>[2x]RPMDNEAVQFGMSMGIGWNLGNQMDAHYDGCSYETGWGNKAATQQTFNG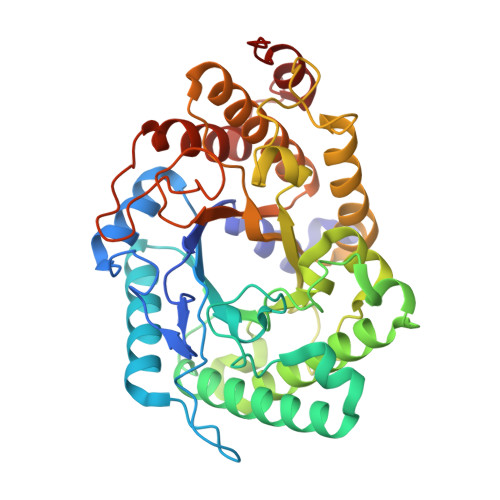LAKAGFRSVRIPVTWMGHIGNAPTYAIERGWLDRVDELVHMAHKAGLIVIINIHHDGFGAADTPSKGSHWLDLPAAVASEERNQLIKQELTMIWLQIGKRFANDGEWLVFETLNEIQDGDWGNGNNRRDGGAQYRVLNEWNQVCVDAIRAAGGKNETRYIGVPGYVCNPDLTVENLVLPEDVVPNRLMVAVHSYDPWDYAGSAKYNEWGHTGKDVVPGVGEEAYVGMLNRLFNMYIRRGVPVYFGEFGAVRRASKADEEFRLYYFRYICKAMRDRRISALYWDNGNSKAGNDGFGVIDHATGRFIGNGEQAVRAMIDSWENNDPNYTLQSIYDSAPESSR> PLSEIPTDDNPNMSMAEMLRRDEGLRLKVYWDTEGYPTIGIGHLIMKQPVRDMAQINKVLSKQVGREITGNPGSITMEEATTLFERDLADMQRDIKSHSKVGPVWQAVNRSRQMALENMAFQMGVGGVAKFNTMLTAMLAGDWEKAYKAGRDSLWYQQTKG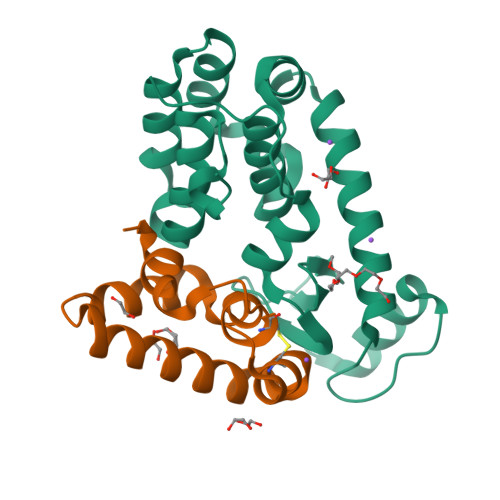RASRVTMIILTGNLESYGVE;> GYDKDLCEWSMTADQTEVETQIEADIMNIVKRDRPEMKAEVQKQLKSGGVMQYNYVLYCDKNFNNKNIIAEVVGE> MGRDICTLDNVYANNLGMLTKLAHVTVPNLYQDAFFSALFAEDSLVAKNKK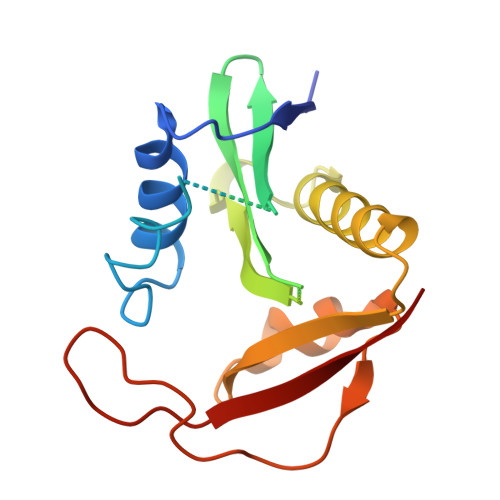PSSKKDVHFTQMAYYSEIPVGGLVAKLVPKKQNELSLKGIQIEFLGVLPNYRHKSIGSKLLKFAEDKCSECHQHNVFVYLPAVDDLTKQWFIAHGFEQVGETVNNFIKGVNGDEQDAILLKKHIS>[3x]MGSSHHHHHHSQDPNSMANPLFRKHIVSINDISRNELELIVKTAAKLKEQPQPELLKNKVIASCFFEAS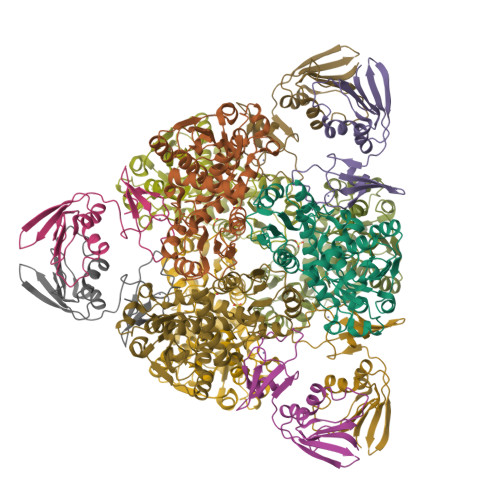TRTRLSFETAIQRLGGSVIGFDNAGNTSLAKKGETLADSISVISSYADAFVMRHPQEGAARLASEFSNVPVINGGDGSNQHPTQTLLDLFSIYETQGRLDNLNIAFVGDLKYGRTVHSLAQALAKFDGCKFHFIAPDALAMPEYICDELDEQNISYATYASIEEVVPEIDVLYMTRVQKERFDETEYQHMKAGFILSASSLVHAKPNLKVLHPLPRVDEIATDVDKTPYAYYFQQAENGVYAREALLALVLNETIGE;>[3x]MKNNHMQVEAICNGYVIDHIPSGQGVKILKLFSLTDTKQRVTVGFNLPTKDGNAKDLIKVENTEITKSQANQLALLAPNATINIIENFKVTDKHSLTLPNEVENVFPCPNSNCITHGEPVTSSFSIKKTKGNIGLKCKYCEKTFSKDIVTEQV>[2x]MDNSHDSDSVFLYHIPCDNCGSSDGNSLFSDGHTFCYVCEKWTAGNEDTKERASKRKPSGGKPGTYNVWNFGESNGRYSALTARGISKETCQKAGYWIAKVDGVMYQVADYRDQNGNIVSQKVRDKDKNFKTTGSHKSDALFGKHLWNGGKKIVVTEGEIDMLTVMELQDCKYPVVSLGHGASAAKKTCAANYEYFDQFEQIIL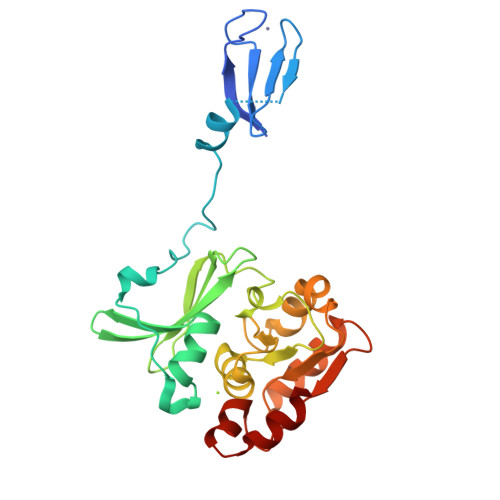MFDMDEAGRKAVEEAAQVLPAGKVRVAVLPCKDANECHLNGHDREIMEQVW>[2x]MSSGKKPVKVKTPAGKEAELVPEKVWAL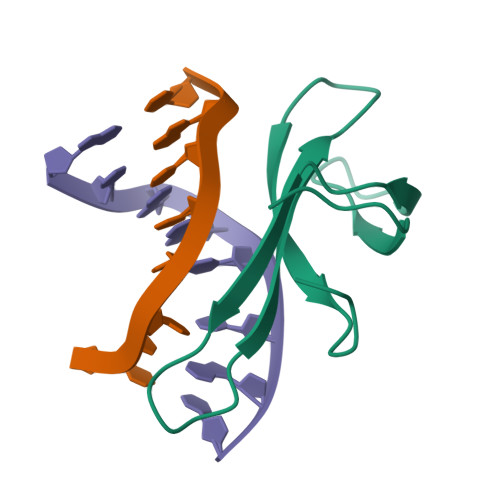APKGRKGVKIGLFKDPETGKYFRHKLPDDYPI>[6x]SSATPIVQFQGESNCLKCFRYRLNDKH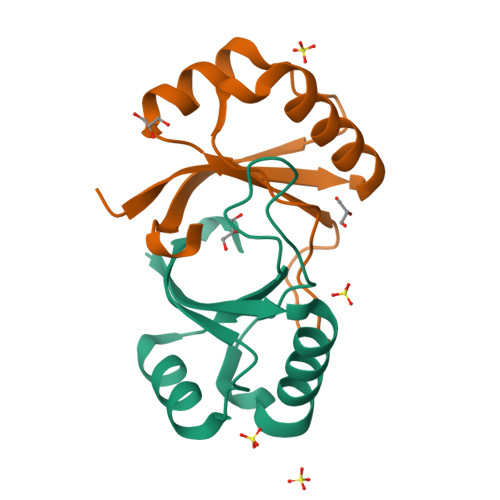RHLFDLISSTWHWASPKAPHKHAIVTVTYHSEEQRQQFLNVVKIPPTIRHKLGFMSMHLL>[2x]MNQHLLGNPKLTVTHVNEVKAGINHIVVDSVQYGNQEMIMEKDGTVEMRDGEKLYINIFRPNKDGKFPVVMSADTYGKDNKPKITNMGALWPTLGTIPTSSFTPEESPDPGFWVPNDYVVVKVALRGSDKSKGVLSPWSKREAEDYYEVIEWAANQSWSNGNIGTNGVSYLAVTQWWVASLNPPHLKAMIPWEGLNDMYREVAFHGGIPDTGFYRFWTQGIFARWTDNPNIEDLIQAQQEHPLFDDFWKQRQVPLSQIKTPLLTCASWSTQGLHNRGSFEGFKQAASEEKWLYVHGRKEWESYYARENLERQKSFFDFYLKEENNDWKDTPHVIYEVRDQFYKGEFKSASAFPLPNAEYTPLYLNAENHTLNHAKISSAHVAQYDSEDKQQDVSFKYTFDKDTELVGNMNLKLWVSTK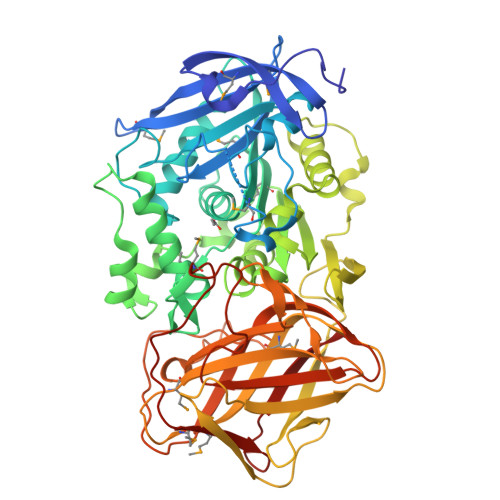DSDDMDLFAGIKKLDRRGNEVNFPDFNHIENGQVATGWLRVSHRELDQEKSSIAQPWHKHETELKLSQDEIVPVEIELLPSGTLFKQGETLEVVVKGSEIVIGNSTPGMKTRYEHEETVNKGMHMIYTGGKYDSQLIIPIVN> IVGGQECKDGECPWQALLINEENEGFCGGTILSEFYILTAAHCLYQAKRFKVRVGDRNTEQEEGGEAVHEVEVVIKHNRFTKETYDFDIAVLRLKTPITFRMNVAPACLPERDWAESTLMTQKTGIVSGFGRTHEKGEQSTRLKMLEVPYVDRNSCKLSSSFIITQNMFCAGYDTKQEDACQGDSGGPHVTRFKDTYFVTGIVSWGEGCARKGKYGIYTKVTAFLKWIDRSMKT;> KLCSLDNGDCDQFCHEEQNSVVCSCARGYTLADNGK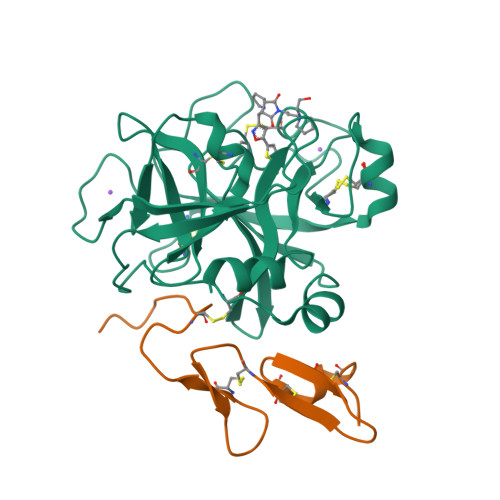ACIPTGPYPCGKQTLERR>[2x]MANIEIPYGKSKLAFDLPDERIQGILRSKAGSYKVNMSEEDIVKRALENPIGTKRLQDLAEGKKNIVIITSDHTRPVPSRITLPLLLDEIRKKNKSANVKILIATGFHRGTTLQEMKAKFGEDLVENEQFVVHDSRNSENMELIGTL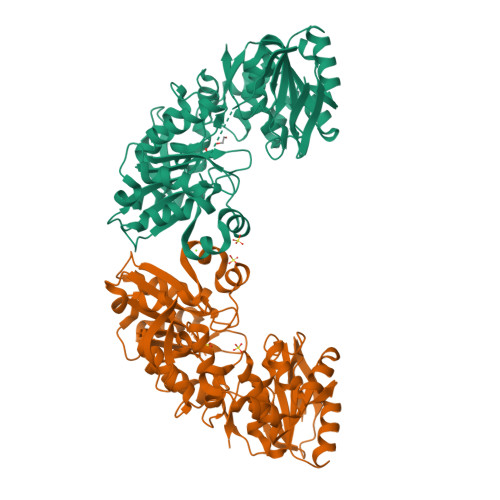PSGGKLEINKLAVEADLLVAEGFIEPHFFAGFSGGRKSILPGIASVQCILANHCSEFIKNPYARTGVLENNPIHRDMIYAAKKANLAFILNVVIDSSHKIVNAFAGHSEKAHLKGCEFVSEIATVNAKPADIVITSNGGYPLDQNIYQSVKGMTAGEAACKDGGVIIIAAECADGHGGEGFYRWFKESKDPQDVMNKILSRGRDETLPDQWEAQILARILINHKVIMVTDSKNYEYVKDMFMTPAKDLGEALKIAESIVNNDSKINVIPDGVSVIVREKASWSHPQFEK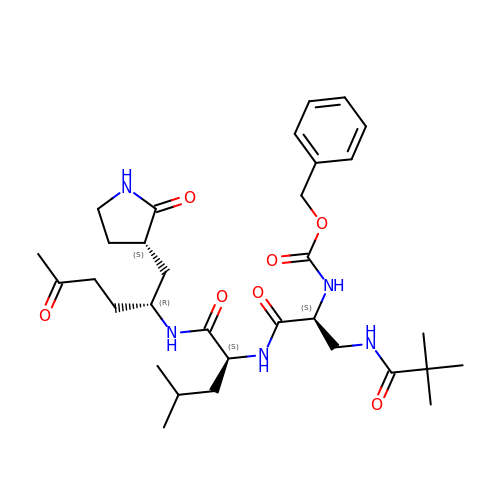N-[(benzyloxy)carbonyl]-3-[(2,2-dimethylpropanoyl)amino]-L-alanyl-N-[(1R)-4-oxo-1-{[(3S)-2-oxopyrrolidin-3-yl]methyl}pentyl]-L-leucinamide | C32 H49 N5 O7 | IEQRDAZPCPYZAJ-QYOOZWMWSA-N The MCM motor of the eukaryotic replicative helicase is loaded as a double hexamer onto DNA by the Origin Recognition Complex (ORC), Cdc6, and Cdt1. ATP binding supports formation of the ORC-Cdc6-Cdt1-MCM (OCCM) helicase-recruitment complex where ORC-Cdc6 and one MCM hexamer form two juxtaposed rings around duplex DNA. MCM is a ring-shaped helicase containing six related AAA+ ATPase polypeptides featuring bipartite active sites with catalytic residues contributed by neighbouring subunits. Biochemical studies established that ATP hydrolysis by MCM, but not ORC or Cdc6, are essential to complete helicase loading.

To better understand the role of ATP hydrolysis during OCCM to SH transition, we employed cryo-EM to analyse the DH loading reaction on MH-capped ARS1 DNA, using MCM-Cdt1 complexes containing the Mcm2RA variant. We solved a 3.3 Å resolution consensus structure and separate local refinements of the ORC-Cdc6 and MCM-Cdt1 regions of the map improved the resolution to 3.2 Å for each sub-volume. Cryo-EM density for all subunits of the ATPγS-OCCM complex could be recognised in OCCMMcm2RA, however, the topologically closed ORC-Cdc6 ring transitions to a notched state, while the notched MCM ring becomes topologically closed. Moreover, cryo-EM density for Cdc6 in OCCMMcm2RA becomes fragmented, reflecting increased flexibility. As a result, duplex DNA appears merely clamped by ORC-Cdc6, and not fully encircled by a protein ring, as observed in ATPγS-OCCM22. The Mcm2RA N-terminal B domain transitions from partially plugging the MCM central channel (ATPγS-OCCM state) to a retracted configuration that creates the space for full access of the double helix into the MCM pore. In fact, continuous cryo-EM density for duplex DNA can be observed spanning the entire length of the MCM ring, unlike ATPγS-OCCM where the double helix is only seen encircled by the ATPase tier. In OCCMMcm2RA, Mcm7 disengages from the ATPase spiral and from DNA, while Mcm2 forms new contacts with the double helix. In OCCMMcm2RA, instead, three sites were ATP bound, while no nucleotide density could be resolved in the Orc1-Cdc6 active site. Within the MCM ATPase, four sites are occupied in ATPγS-OCCM, while all active sites are nucleotide-bound in the six MCM subunits of OCCMMcm2RA.

> MSDNRRRRREEDDSDSENELPPSSPQQHFRGGMNPVSSPIGSPDMINPEGDDNEVDDVPDIDEVEEQMNEVDLMDDNMYEDYAADHNRDRYDPDQVDDREQQELSLSERRRIDAQLNERDRLLRNVAYIDDEDEEQEGAAQLDEMGLPVQRRRRRRQYEDLENSDDDLLSDMDIDPLREELTLESLSNVKANSYSEWITQPNVSRTIARELKSFLLEYTDETGRSVYGARIRTLGEMNSESLEVNYRHLAESKAILALFLAKCPEEMLKIFDLVAMEATELHYPDYARIHSEIHVRISDFPTIYSLRELRESNLSSLVRVTGVVTRRTGVFPQLKYVKFNCLKCGSILGPFFQDSNEEIRISFCTNCKSKGPFRVNGEKTVYRNYQRVTLQEAPGTVPPGRLPRHREVILLADLVDVSKPGEEVEVTGIYKNNYDGNLNAKNGFPVFATIIEANSIKRREGNTANEGEEGLDVFSWTEEEEREFRKISRDRGIIDKIISSMAPSIYGHRDIKTAVACSLFGGVPKNVNGKHSIRGDINVLLLGDPGTAKSQILKYVEKTAHRAVFATGQGASAVGLTASVRKDPITKEWTLEGGALVLADKGVCLIDEFDKMNDQDRTSIHEAMEQQSISISKAGIVTTLQARCSIIAAANPNGGRYNSTLPLAQNVSLTEPILSAFDILCVVRDLVDEEADERLATFVVDSHVRSHPENDEDREGEELKNNGESAIEQGEDEINEQLNARQRRLQRQRKKEEEISPIPQELLMKYIHYARTKIYPKLHQMDMDKVSRVYADLRRESISTGSFPITVRHLESILRIAESFAKMRLSEFVSSYDLDRAIKVVVDSFVDAQKVSVRRQLRRSFAIYTLGH;> MKRRWKKNFIAVSAANRFKKISSSGALENLYFQGEMEGSTGFDGDATTFFAPDAVFGDRVRRFQEFLDTFTSYRDSVRSIQVYNSNNAANYNDDQDDADERDLLGDDDGDDLEKEKKAASSTSLNILPHRIIISLDDLREFDRSFWSGILVEPAYFIPPAEKALTDLADSMDDVPHPNASAVSSRHPWKLSFKGSFGAHALSPRTLTAQHLNKLVSVEGIVTKTSLVRPKLIRSVHYAAKTGRFHYRDYTDATTTLTTRIPTPAIYPTEDTEGNKLTTEYGYSTFIDHQRITVQEMPEMAPAGQLPRSIDVILDDDLVDKTKPGDRVNVVGVFKSLGAGGMNQSNSNTLIGFKTLILGNTVYPLHARSTGVAARQMLTDFDIRNINKLSKKKDIFDILSQSLAPSIYGHDHIKKAILLMLMGGVEKNLENGSHLRGDINILMVGDPSTAKSQLLRFVLNTASLAIATTGRGSSGVGLTAAVTTDRETGERRLEAGAMVLADRGVVCIDEFDKMTDVDRVAIHEVMEQQTVTIAKAGIHTTLNARCSVIAAANPVFGQYDVNRDPHQNIALPDSLLSRFDLLFVVTDDINEIRDRSISEHVLRTHRYLPPGYLEGEPVRERLNLSLAVGEDADINPEEHSNSGAGVENEGEDDEDHVFEKFNPLLQAGAKLAKNKGNYNGTEIPKLVTIPFLRKYVQYAKERVIPQLTQEAINVIVKNYTDLRNDDNTKKSPITARTLETLIRLATAHAKVRLSKTVNKVDAKVAANLLRFALLGEDIGNDIDEEESEYEEALSKRSPQKSPKKRQRVRQPASNSGSPIKSTPRRSTASSVNATPSSARRILRFQDDEQNAGEDDNDIMSPLPADEEAELQRRLQLGLRVSPRRREHLHAPEEGSSGPLTEVGTPRLPNVSSAGQDDEQQQSVISFDNVEPGTISTGRLSLISGIIARLMQTEIFEEESYPVASLFERINEELPEEEKFSAQEYLAGLKIMSDRNNLMVADDKVWRV;> MSQQSSSPTKEDNNSSSPVVPNPDSVPPQLSSPALFYSSSSSQGDIYGRNNSQNLSQGEGNIRAAIGSSPLNFPSSSQRQNSDVFQSQGRQGRIRSSASASGRSRYHSDLRSDRALPTSSSSLGRNGQNRVHMRRNDIHTSDLSSPRRIVDFDTRSGVNTLDTSSSSAPPSEASEPLRIIWGTNVSIQECTTNFRNFLMSFKYKFRKILDEREEFINNTTDEELYYIKQLNEMRELGTSNLNLDARNLLAYKQTEDLYHQLLNYPQEVISIMDQTIKDCMVSLIVDNNLDYDLDEIETKFYKVRPYNVGSCKGMRELNPNDIDKLINLKGLVLRSTPVIPDMKVAFFKCNVCDHTMAVEIDRGVIQEPARCERIDCNEPNSMSLIHNRCSFADKQVIKLQETPDFVPDGQTPHSISLCVYDELVDSCRAGDRIEVTGTFRSIPIRANSRQRVLKSLYKTYVDVVHVKKVSDKRLDVDTSTIEQELMQNKVDHNEVEEVRQITDQDLAKIREVAAREDLYSLLARSIAPSIYELEDVKKGILLQLFGGTNKTFTKGGRYRGDINILLCGDPSTSKSQILQYVHKITPRGVYTSGKGSSAVGLTAYITRDVDTKQLVLESGALVLSDGGVCCIDEFDKMSDSTRSVLHEVMEQQTISIAKAGIITTLNARSSILASANPIGSRYNPNLPVTENIDLPPPLLSRFDLVYLVLDKVDEKNDRELAKHLTNLYLEDKPEHISQDDVLPVEFLTMYISYAKEHIHPIITEAAKTELVRAYVGMRKMGDDSRSDEKRITATTRQLESMIRLAEAHAKMKLKNVVELEDVQEAVRLIRSAIKDYATDPKTGKIDMNLVQTGKSVIQRKLQEDLSREIMNVLKDQASDSMSFNELIKQINEHSQDRVESSDIQEALSRLQQEDKVIVLGEGVRRSVRLNNRV;> MSFDRPEIYSAPVLQGESPNDDDNTEIIKSFKNFILEFRLDSQFIYRDQLRNNILVKNYSLTVNMEHLIGYNEDIYKKLSDEPSDIIPLFETAITQVAKRISILSRAQSANNNDKDPENTSMDTDSLLLNSLPTFQLILNSNANQIPLRDLDSEHVSKIVRLSGIIISTSVLSSRATYLSIMCRNCRHTTSITINNFNSITGNTVSLPRSCLSTIESESSMANESNIGDESTKKNCGPDPYIIIHESSKFIDQQFLKLQEIPELVPVGEMPRNLTMTCDRYLTNKVIPGTRVTIVGIYSIYNSKNGAGSGRSGGGNGGSGVAIRTPYIKILGIQSDVETSSIWNSVTMFTEEEEEEFLQLSRNPKLYEILTNSIAPSIFGNEDIKKAIVCLLMGGSKKILPDGMRLRGDINVLLLGDPGTAKSQLLKFVEKVSPIAVYTSGKGSSAAGLTASVQRDPMTREFYLEGGAMVLADGGVVCIDEFDKMRDEDRVAIHEAMEQQTISIAKAGITTVLNSRTSVLAAANPIYGRYDDLKSPGDNIDFQTTILSRFDMIFIVKDDHNEERDISIANHVINIHTGNANAMQNQQEENGSEISIEKMKRYITYCRLKCAPRLSPQAAEKLSSNFVTIRKQLLINELESTERSSIPITIRQLEAIIRITESLAKLELSPIAQERHVDEAIRLFQASTMDAASQDPIGGLNQASGTSLSEIRRFEQELKRRLPIGWSTSYQTLRREFVDTHRFSQLALDKALYALEKHETIQLRHQGQNIYRSGV;> MSSPFPADTPSSNRPSNSSPPPSSIGAGFGSSSGLDSQIGSRLHFPSSSQPHVSNSQTGPFVNDSTQFSSQRLQTDGSATNDMEGNEPARSFKSRALNHVKKVDDVTGEKVREAFEQFLEDFSVQSTDTGEVEKVYRAQIEFMKIYDLNTIYIDYQHLSMRENGALAMAISEQYYRFLPFLQKGLRRVVRKYAPELLNTSDSLKRSEGDEGQADEDEQQDDDMNGSSLPRDSGSSAAPGNGTSAMATRSITTSTSPEQTERVFQISFFNLPTVHRIRDIRSEKIGSLLSISGTVTRTSEVRPELYKASFTCDMCRAIVDNVEQSFKYTEPTFCPNPSCENRAFWTLNVTRSRFLDWQKVRIQENANEIPTGSMPRTLDVILRGDSVERAKPGDRCKFTGVEIVVPDVTQLGLPGVKPSSTLDTRGISKTTEGLNSGVTGLRSLGVRDLTYKISFLACHVISIGSNIGASSPDANSNNRETELQMAANLQANNVYQDNERDQEVFLNSLSSDEINELKEMVKDEHIYDKLVRSIAPAVFGHEAVKKGILLQMLGGVHKSTVEGIKLRGDINICVVGDPSTSKSQFLKYVVGFAPRSVYTSGKASSAAGLTAAVVRDEEGGDYTIEAGALMLADNGICCIDEFDKMDISDQVAIHEAMEQQTISIAKAGIHATLNARTSILAAANPVGGRYNRKLSLRGNLNMTAPIMSRFDLFFVILDDCNEKIDTELASHIVDLHMKRDEAIEPPFSAEQLRRYIKYARTFKPILTKEARSYLVEKYKELRKDDAQGFSRSSYRITVRQLESMIRLSEAIARANCVDEITPSFIAEAYDLLRQSIIRVDVDDVEMDEEFDNIESQSHAASGNNDDNDDGTGSGVITSEPPADIEEGQSEATARPGTSEKKKTTVTYDKYVSMMNMIVRKIAEVDREGAEELTAVDIVDWYLLQKENDLGSLAEYWEERRLAFKVIKRLVKDRILMEIHGTRHNLRDLENEENENNKTVYVIHPNCEVLDQLEPQDSS;> MSAALPSIQLPVDYNNLFNEITDFLVTFKQDTLSSDATRNENEDENLDAENIEQHLLEKGPKYMAMLQKVANRELNSVIIDLDDILQYQNEKFLQGTQADDLVSAIQQNANHFTELFCRAIDNNMPLPTKEIDYKDDVLDVILNQRRLRNERMLSDRTNEIRSENLMDTTMDPPSSMNDALREVVEDETELFPPNLTRRYFLYFKPLSQNCARRYRKKAISSKPLSVRQIKGDFLGQLITVRGIITRVSDVKPAVEVIAYTCDQCGYEVFQEVNSRTFTPLSECTSEECSQNQTKGQLFMSTRASKFSAFQECKIQELSQQVPVGHIPRSLNIHVNGTLVRSLSPGDIVDVTGIFLPAPYTGFKALKAGLLTETYLEAQFVRQHKKKFASFSLTSDVEERVMELITSGDVYNRLAKSIAPEIYGNLDVKKALLLLLVGGVDKRVGDGMKIRGDINVCLMGDPGVAKSQLLKAICKISPRGVYTTGKGSSGVGLTAAVMKDPVTDEMILEGGALVLADNGICCIDEFDKMDESDRTAIHEVMEQQTISISKAGINTTLNARTSILAAANPLYGRYNPRLSPLDNINLPAALLSRFDILFLMLDIPSRDDDEKLAEHVTYVHMHNKQPDLDFTPVEPSKMREYIAYAKTKRPVMSEAVNDYVVQAYIRLRQDSKREMDSKFSFGQATPRTLLGIIRLSQALAKLRLADMVDIDDVEEALRLVRVSKESLYQETNKSKEDESPTTKIFTIIKKMLQETGKNTLSYENIVKTVRLRGFTMLQLSNCIQEYSYLNVWHLINEGNTLKFVDDGTMDTDQEDSLVSTPKLAPQTTASANVSAQDSDIDLQDA;> MSGTANSRRKEVLRVPVIDLNRVSDEEQLLPVVRAILLQHDTFLLKNYANKAVLDALLAGLTTKDLPDTSQGFDANFTGTLPLEDDVWLEQYIFDTDPQLRFDRKCRNESLCSIYSRLFKLGLFFAQLCVKSVVSSAELQDCISTSHYATKLTRYFNDNGSTHDGADAGATVLPTGDDFQYLFERDYVTFLPTGVLTIFPCAKAIRYKPSTMATTDNSWVSIDEPDCLLFHTGTLLARWSQGMHTTSPLQIDPRANIVSLTIWPPLTTPISSKGEGTIANHLLEQQIKAFPKVAQQYYPRELSILRLQDAMKFVKELFTVCETVLSLNALSRSTGVPPELHVLLPQISSMMKRKIVQDDILKLLTIWSDAYVVELNSRGELTMNLPKRDNLTTLTNKSRTLAFVERAESWYQQVIASKDEIMTDVPAFKINKRRSSSNSKTVLSSKVQTKSSNANALNNSRYLANSKENFMYKEKMPDSQANLMDRLRERERRSAALLSQRQKRYQQFLAMKMTQVFDILFSLTRGQPYTETYLSSLIVDSLQDSNNPIGTKEASEILAGLQGILPMDISVHQVDGGLKVYRWNSLDKNRFSKLLQIHKSKQQD;> MKRRWKKNFIAVSAANRFKKISSSGALENLYFQGEMAKTLKDLQGWEIITTDEQGNIIDGGQKRLRRRGAKTEHYLKRSSDGIKLGRGDSVVMHNEAAGTYSVYMIQELRLNTLNNVVELWALTYLRWFEVNPLAHYRQFNPDANILNRPLNYYNKLFSETANKNELYLTAELAELQLFNFIRVANVMDGSKWEVLKGNVDPERDFTVRYICEPTGEKFVDINIEDVKAYIKKVEPREAQEYLKDLTLPSKKKEIKRGPQKKDKATQTAQISDAETRATDITDNEDGNEDESSDYESPSDIDVSEDMDSGEISADELEEEEDEEEDEDEEEKEARHTNSPRKRGRKIKLGKDDIDASVQPPPKKRGRKPKDPSKPRQMLLISSCRANNTPVIRKFTKKNVARAKKKYTPFSKRFKSIAAIPDLTSLPEFYGNSSELMASRFENKLKTTQKHQIVETIFSKVKKQLNSSYVKEEILKSANFQDYLPARENEFASIYLSAYSAIESDSATTIYVAGTPGVGKTLTVREVVKELLSSSAQREIPDFLYVEINGLKMVKPTDCYETLWNKVSGERLTWAASMESLEFYFKRVPKNKKKTIVVLLDELDAMVTKSQDIMYNFFNWTTYENAKLIVIAVANTMDLPERQLGNKITSRIGFTRIMFTGYTHEELKNIIDLRLKGLNDSFFYVDTKTGNAILIDAAGNDTTVKQTLPEDVRKVRLRMSADAIEIASRKVASVSGDARRALKVCKRAAEIAEKHYMAKHGYGYDGKTVIEDENEEQIYDDEDKDLIESNKAKDDNDDDDDNDGVQTVHITHVMKALNETLNSHVITFMTRLSFTAKLFIYALLNLMKKNGSQEQELGDIVDEIKLLIEVNGSNKFVMEIAKTLFQQGSDNISEQLRIISWDFVLNQLLDAGILFKQTMKNDRICCVKLNISVEEAKRAMNEDETLRNL;> MLNGEDFVEHNDILSSPAKSRNVTPKRVDPHGERQLRRIHSSKKNLLERISLVGNERKNTSPDPALKPKTPSKAPRKRGRPRKIQEELTDRIKKDEKDTISSKKKRKLDKDTSGNVNEESKTSNNKQVMEKTGIKEKREREKIQVATTTYEDNVTPQTDDNFVSNSPEPPEPATPSKKSLTTNHDFTSPLKQIIMNNLKEYKDSTSPGKLTLSRNFTPTPVPKNKKLYQTSETKSASSFLDTFEGYFDQRKIVRTNAKSRHTMSMAPDVTREEFSLVSNFFNENFQKRPRQKLFEIQKKMFPQYWFELTQGFSLLFYGVGSKRNFLEEFAIDYLSPKIAYSQLAYENELQQNKPVNSIPCLILNGYNPSCNYRDVFKEITDLLVPAELTRSETKYWGNHVILQIQKMIDFYKNQPLDIKLILVVHNLDGPSIRKNTFQTMLSFLSVIRQIAIVASTDHIYAPLLWDNMKAQNYNFVFHDISNFEPSTVESTFQDVMKMGKSDTSSGAEGAKYVLQSLTVNSKKMYKLLIETQMQNMGNLSANTGPKRGTQRTGVELKLFNHLCAADFIASNEIALRSMLREFIEHKMANITKNNSGMEIIWVPYTYAELEKLLKTVLNTL;> MSDLNQSKKMNVSEFADAQRSHYTVYPSLPQSNKNDKHIPFVKLLSGKESEVNVEKRWELYHQLHSHFHDQVDHIIDNIEADLKAEISDLLYSETTQKRRCFNTIFLLGSDSTTKIELKDESSRYNVLIELTPKESPNVRMMLRRSMYKLYSAADAEEHPTIKYEDINDEDGDFTEQNNDVSYDLSLVENFKRLFGKDLAMVFNFKDVDSINFNTLDNFIILLKSAFKYDHVKISLIFNINTNLSNIEKNLRQSTIRLLKRNYHKLDVSSNKGFKYGNQIFQSFLDTVDGKLNLSDRFVEFILSKMANNTNHNLQLLTKMLDYSLMSYFFQNAFSVFIDPVNVDFLNDDYLKILSRCPTFMFFVEGLIKQHAPADEILSLLTNKNRGLEEFFVEFLVRENPINGHAKFVARFLEEELNITNFNLIELYHNLLIGKLDSYLDRWSACKEYKDRLHFEPIDTIFQELFTLDNRSGLLTQSIFPSYKSNIEDNLLSWEQVLPSLDKENYDTLSGDLDKIMAPVLGQLFKLYREANMTINIYDFYIAFRETLPKEEILNFIRKDPSNTKLLELAETPDAFDKVALILFMQAIFAFENMGLIKFQSTKSYDLVEKCVWRGI;> MTISEARLSPQVNLLPIKRHSNEEVEETAAILKKRTIDNEKCKDSDPGFGSLQRRLLQQLYGTLPTDEKIIFTYLQDCQQEIDRIIKQSIIQKESHSVILVGPRQSYKTYLLDYELSLLQQSYKEQFITIRLNGFIHSEQTAINGIATQLEQQLQKIHGSEEKIDDTSLETISSGSLTEVFEKILLLLDSTTKTRNEDSGEVDRESITKITVVFIFDEIDTFAGPVRQTLLYNLFDMVEHSRVPVCIFGCTTKLNILEYLEKRVKSRFSQRVIYMPQIQNLDDMVDAVRNLLTVRSEISPWVSQWNETLEKELSDPRSNLNRHIRMNFETFRSLPTLKNSIIPLVATSKNFGSLCTAIKSCSFLDIYNKNQLSNNLTGRLQSLSDLELAILISAARVALRAKDGSFNFNLAYAEYEKMIKAINSRIPTVAPTTNVGTGQSTFSIDNTIKLWLKKDVKNVWENLVQLDFFTEKSAVGLRDNATAAFYASNYQFQGTMIPFDLRSYQMQIILQELRRIIPKSNMYYSWTQL;> MNVTTPEVAFREYQTNCLASYISADPDITPSNLILQGYSGTGKTYTLKKYFNANPNLHAVWLEPVELVSWKPLLQAIARTVQYKLKTLYPNIPTTDYDPLQVEEPFLLVKTLHNIFVQYESLQEKTCLFLILDGFDSLQDLDAALFNKYIKLNELLPKDSKINIKFIYTMLETSFLQRYSTHCIPTVMFPRYNVDEVSTILVMSRCGELMEDSCLRKRIIEEQITDCTDDQFQNVAANFIHLIVQAFHSYTGNDIFALNDLIDFKWPKYVSRITKENIFEPLALYKSAIKLFLSTDDNLSENGQGESAITTNRDDLENSQTYDLSIISKYLLIASYICSYLEPRYDASIFSRKTRIIQGRAAYGRRKKKEVNPRYLQPSLFAIERLLAIFQAIFPIQGKAESGSLSALREESLMKANIEVFQNLSELHTLKLIATTMNKNIDYLSPKVRWKVNVPWEIIKEISESVHFNISDYFSDIHE;> MSMQQVQHCVAEVLRLDPQEKPDWSSGYLKKLTNATSILYNTSLNKVMLKQDEEVARCHICAYIASQKMNEKHMPDLCYYIDSIPLEPKKAKHLMNLFRQSLSNSSPMKQFAWTPSPKKNKRSPVKNGGRFTSSDPKELRNQLFGTPTKVRKSQNNDSFVIPELPPMQTNESPSITRRKLAFEEDEDEDEEEPGNDGLSLKSHSNKSITGTRNVDSDEYENHESDPTSEEEPLGVQESRSGRTKQNKAVGKPQSELKTAKALRKRGRIPNSLLVKKYCKMTTEEIIRLCNDFELPREVAYKIVDEYNINASRLVCPWQLVCGLVLNCTFIVFNERRRKDPRIDHFIVSKMCSLMLTSKVDDVIECVKLVKELIIGEKWFRDLQIRYDDFDGIRYDEIIFRKLGSMLQTTNILVTDDQYNIWKKRIEMDLALTEPL> GIITCICDLNDDDGFTIQCDHC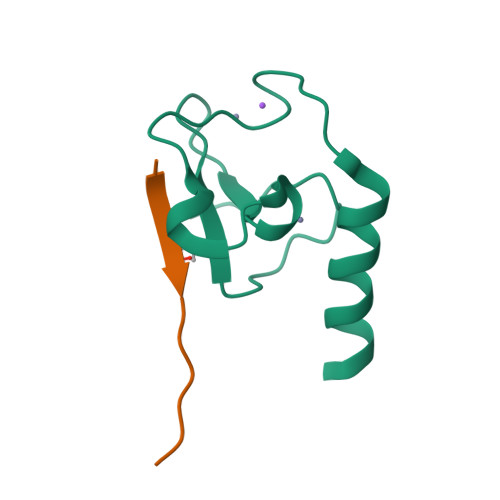NRWQHAICYGIKDIGMAPDDYLCNSCDPREVDINLARKIQQERINVK;> ARTKQTARKST>MAEKRTVRPFAGTERRAKGWI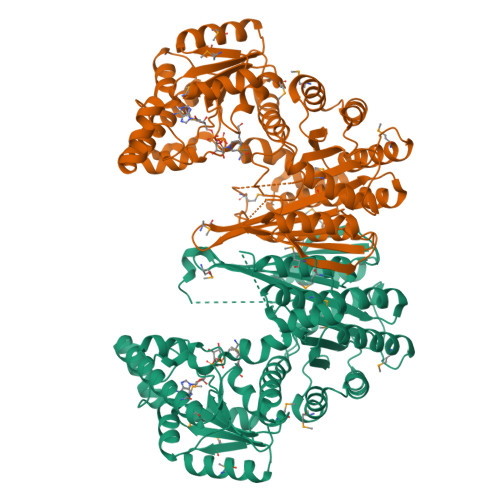QEAALRMLNNNLHPDVAERPDELIVYGGIGKAARNWECYEAIVDTLLRLENDETLLIQSGKPVAVFRTHPDAPRVLIANSNLVPAWATWDHFHELDKKGLIMYGQMTAGSWIYIGSQGIVQGTYETFAEVARQHFGGTLAGTITLTAGLGGMGGAQPLAVTMNGGVCLAIEVDPARIQRRIDTNYLDTMTDSLDAALEMAKQAKEEKKALSIGLVGNAAEVLPRLVETGFVPDVLTDQTSAHDPLNGYIPAGLTLDEAAELRARDPKQYIARAKQSIAAHVRAMLAMQKQGAVTFDYGNNIRQVAKDEGVDDAFSFPGFVPAYIRPLFCEGKGPFRWVALSGDPEDIYKTDEVILREFSDNERLCHWIRMAQKRIKFQGLPARICWLGYGERAKFGKIINDMVAKGELKAPIVIGRDHLDSGSVASPNRETEGMKDGSDAIADWPILNALLNAVGGASWVSVHHGGGVGMGYSIHAGMVIVADGTKEAEKRLERVLTTDPGLGVIRHADAGYELAIRTAKEKGIDMPMLK[2x]> MQVNRLPFFTNHFFDTYLLISEDTPVGSSVTQLLARDMDNDPLVFGVSGEEASRFFAVEPDTGVVWLRQPLDRETKSEFTVEFSVSDHQGVITRKVNIQVGDVNDNAPTFHNQPYSVRIPENTPVGTPIFIVNATDPDLGAGGSVLYSFQPPSPFFAIDSARGIVTVIQELDYEVTQAYQLTVNATDQDKTRPLSTLANLAIIITDLEHHHHHH;> MQYDDDWQYEDCKLARGGPPATIVAIDEESRNGTILVDNMLIKGTAGGPDPTIELSLKDNVDYWVLLDPVKQMLFLN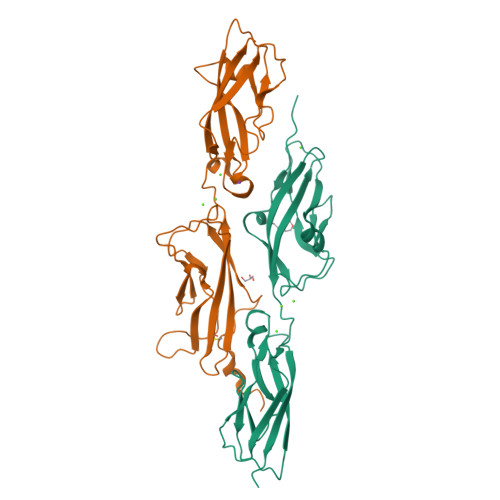STGRVLDRDPPMNIHSIVVQVQCVNKKVGTVIYHEVRIVVRDRNDNSPTFKHESYYATVNELTPVGTTIFTGFSGDNGATDIDDGPNGQIEYVIQYNPEDPTSNDTFEIPLMLTGNVVLRKRLNYEDKTRYYVIIQANDRAQNLNERRTTTTTLTVDLEHHHHHH>TLHKERRIGRLSVLLLLNEAEESTQVEELERDGWKVCLGKVGSMDAHKVIAAIETASKKSGVI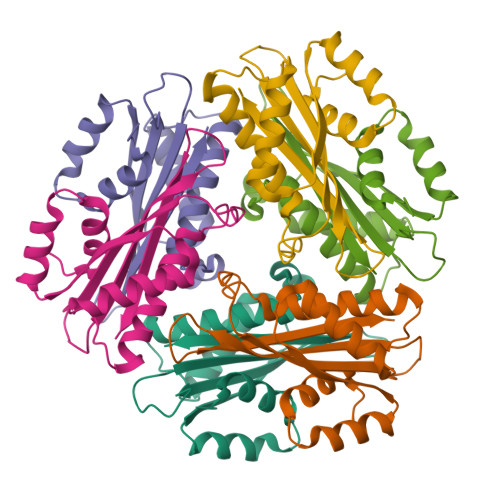QSEGYRESHALYHATMEALHGVTRGEMLLGSLLRTVGLRFAVLRGNPYESEAEGDWIAVSLYGTIGAPIKGLEHETFGVGINHI[2x]> ADTVTLPFANGERPLVMYPGKRPLIGLTARPPQLETPFSVFDEGLITPNDAFFVRYHLAGIPLEIDPDAF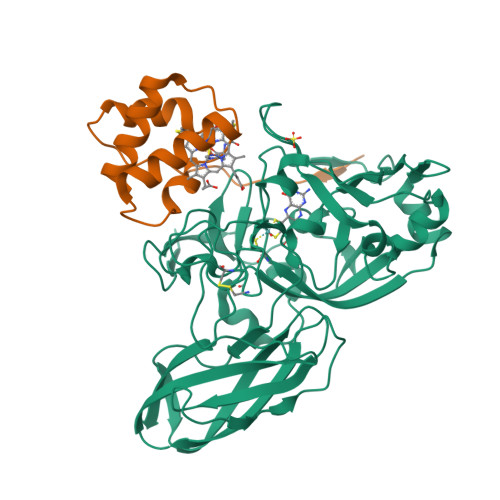RLEIKGKVGTPLSLSLQDLKNDFPASEVVAVNQCSGNSRGFVEPRVGGGQLANGAMGNARWRGVPLKAVLEKAGVQAGAKQVTFGGLDGPVIPETPDFVKALSIDHATDGEVMLAYSMNGADLPWLNGYPLRLVVPGYYGTYWVKHLNEITVIDKEFDGFWMKTAFRIPDNACACTEPGKAPTATIPINRFDVRSFITNVENGASVKAGEVPLRGIAFDGGYGITQVSVSADAGKSWTNATLDPGLGKYSFRGWKAVLPLTKGDHVLMCRATNARGETQPMQATWNPAGYMRNVVEATRVIAA;> APLTYELPDETAQLKPAPQPGFEAAQNNCAACHSVDYINTQPPGKGQAFWDAEVQKMIKVYHAPVDEADAKAIADYLAKTY>[2x]APMSLIKPEMKIKLLMEGNVNGHQFVIEGDGKGHPFEGKQSMDLVVKEGAPLPFAYDILTTAFHYGNRVFAKYPDHIPDYF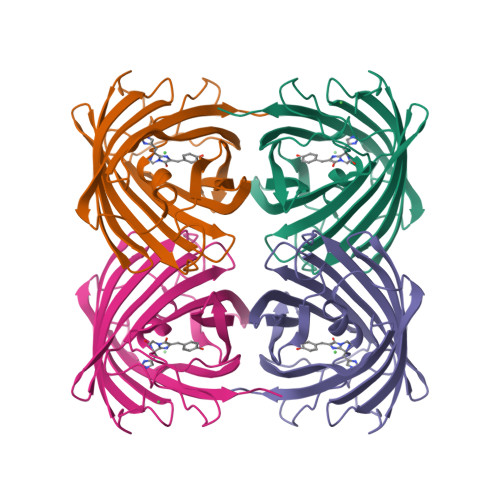KQSFPKGFSWERSLMFEDGGVCIATNDITLKGDTFFNKVRFDGVNFPPNGPVMQKKTLKWEASTEKMYLRDGVLTGDITMALLLKGDVHYRCDFRTTYKSRQEGVKLPGYHFVDHCISILRHDKDYNEVKLYEHAVAHSGLPDNVK>[2x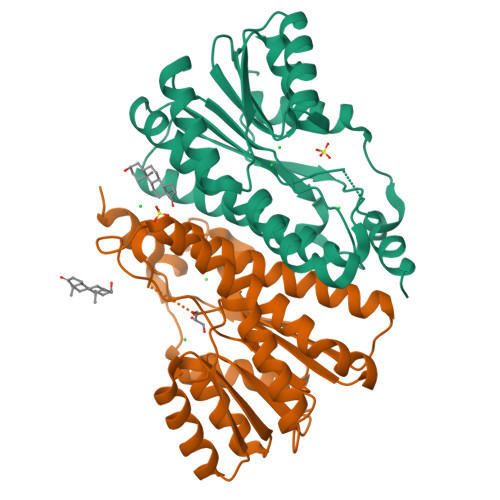]GSSHHHHHHSSGRENLYFQGHMPKRRKSVTGEIVLITGAGHGIGRLTAYEFAKLKSKLVLWDINKHGLEETAAKCKGLGAKVHTFVVDCSNREDIYSSAKKVKAEIGDVSILVNNAGVVYTSDLFATQDPQIEKTFEVNVLAHFWTTKAFLPAMTKNNHGHIVTVASAAGHVSVPFLLAYCSSKFAAVGFHKTLTDELAALQITGVKTTCLCPNFVNTGFIKNPSTSLGPTLEPEEVVNRLMHGILTEQKMIFIPSSIAFLTTLERILPEGS>[2x]MSEQSYRSAGTLLAQLASGETTSVALVNHYFSRMAQFNKPLNAVVQQHYALALEAAARADRERLEGRARGVLHGLPCTVKESFDVQGWLTTSGAHYLKDNRATQDAPSIARLRAAGAILMGKTNVPMMTADWQTYNDLYGTTHNLWDRQRSPGGSSGGAAVAVAADFTPVEFGSDLFGSLRIPAHYTGVYAHRCSLGLMSVRGHVPGGGPQATDEPDLSTAGPMARSAADLRLMMRALSTFWVEPPRIPDFSRYQAKANYRVCTWFSAPHHEIDQQIAQRFQSFIDKLRAQPGVEVDDAMPADIDPDALFDIAVKLSGRLVSTALNGRQRLTAGLAALGFRLVGKLADVPEGITSYYQGMLKDSGEQRNTDKLRHEYSRVIETLFARYDVLLTPVSPVLAFAHMQQPVRKRKLIVNGEPQDYNEHLFWNMLATVFGLPATVYPLAKTMDELPCGIQIISGHFHDDVTINFAEFCESISGGFTVPEGYG

Colibactin is a genotoxic natural product produced by select commensal bacteria in the human gut microbiota. An amidase, ClbL, plays a key role in the pathway, catalyzing the final step in the formation of the pseudodimeric scaffold. ClbL couples α-aminoketone and β-ketothioester intermediates attached to separate carrier domains on the NRPS–PKS assembly. ClbL is a member of the diverse amidase superfamily (AS) of enzymes that are characterized by a highly conserved Ser–cis-Ser–Lys catalytic triad that is key to amide hydrolysis.

ClbL crystallized as a homodimer (space group C121) and a single polypeptide chain consists of 487 residues. Interpretable electron density for residues 318–367 and 208–214 is missing, suggesting flexible loop regions adjacent to and covering the active site. The overall structure displays a compact mixed α/β fold consisting of 12 α-helices and 12 β-strands. Compared with other members of the AS superfamily, a notable structural feature of ClbL is the presence of several disordered regions around the active site. A lack of electron density is evident in both monomers of the asymmetric unit, suggesting that the disordered loops are relevant to the protein in solution. The protein crystallized in an active conformation, as is evident from the covalent conjugation of an unanticipated small molecule to Ser179 in the active site. PMSF, which is present in the ClbL purification steps, models well into the orphan electron density. Electron density corresponding to the phenyl group is not clear, suggesting disorder/nonspecific interactions. Both O atoms of the sulfonate group make hydrogen-bonding interactions with the side-chain hydroxyl of Ser155 and the cis-amide N atom of Ser155.Aurora A kinase is one of the key regulators of mitotic events, including mitotic entry, centrosome maturation and spindle formation, as well as assisting in neuronal migration. Aurora A has attracted significant attention for the development of targeted agents for cancer because it is overexpressed in a wide range of tumors, including breast, colon, ovary and skin malignancies. We note that in Aurora kinase sequences a tryptophan residue, Trp277, is immediately following the DFG motif and displays a drastically different orientation whether Aurora A is in an active (DFG-in) or inactive (DFG-out) conformation. This Trp moiety is unique for the Aurora kinase family in the Ser/Thr kinome and its position is suggested to be important for tuning the substrate specificity.

A plethora of X-ray structures and functional assays led to the general notion that dephosphorylated Aurora A and, more universally, Ser/Thr kinases are in an inactive conformation and that phosphorylation or activator binding induces the active structure. Our results are consistent with other crystallographic studies on wild-type, dephosphorylated Aurora A in its apo or nucleotide bound state, where the kinase was also found in the active conformation (Gustafson et al., 2014; Janeček et al., 2016; Nowakowski et al., 2002). The following observations support our hypothesis: (i) two crystal structures for the apo-protein show Trp277 in very different environments, (ii) Danusertib has been proposed to selectively bind to the DFG-out conformation based on a co-crystal structure, and (iii) the same slow step is observed for binding of both Gleevec and Danusertib. The broad line shape for the Trp277 peak hints at severe exchange broadening in the surrounding of the DFG-loop and is consistent with the high B-factors for Trp277 and its neighboring residues observed in all crystal structures described here. The number of crystals for each structure is one for apo-Aurora A and Aurora A + AMPPCP and two crystals for Aurora A + Mb + AT9283.

> SVDESKKRQWALEDFEIGRPLGKGKFGNVYLAREKQSKFILALKVLFKAQLEKAGVEHQLRREVEIQSHLRHPNILRLYGYFHDATRVYLILEYAPLGTVYRELQKLSKFDEQRTATYITELANALSYCHSKRVIHRDIKPENLLLGSAGELKIADFGWSVHAPSSRRTTLCGTLDYLPPEMIEGRMHDEKVDLWSLGVLCYEFLVGKPPFEANTYQETYKRISRVEFTFPDFVTEGARDLISRLLKHNPSQRPMLREVLEHPWITANSSKPSNCQNKESASKQS>[2x]MVGLLPITAALAATVLPNIVSAVGLDQAAVAKGLQYFGTATDNPELTDIPYVTQLNNTADFGQITPGNSMKWDATEPSQGTFTFTKGDVIADLAEGNGQYLRCHTLVWYNQLPSWVTSGTWTNATLTAALKNHITNVVSHYKGKCLHWDVVNEALNDDGTYRTNIFYTTIGEAYIPIAFAAAAAADPDAKLFYNDYNLEYGGAKAASARAIVQLVKNA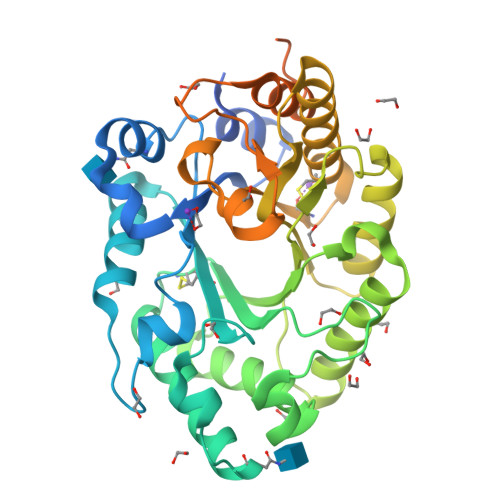GAKIDGVGLQAHFSVGTVPSTSSLVSVLQSFTALGVEVAYTEADVRILLPTTATTLAQQSSDFQALVQSCVQTTGCVGFTIWDWTDKYSWVPSTFSGYGAALPWDENLVKKPAYNGLLAGMGVTVTTTTTTTTATATGKTTTTTAGAASTGTTAAHWGQCGGLNWSGPTVCASGYTCTYVNDYYSQCL N-[(1R)-1-(4-fluorophenyl)ethyl]-N'-[(2S,3S)-3-hydroxy-4-{4-[(1S)-1-hydroxyethyl]-1H-1,2,3-triazol-1-yl}-1-phenylbutan-2-yl]-5-[methyl(methylsulfonyl)amino]benzene-1,3-dicarboxamide | C32 H37 F N6 O6 S | 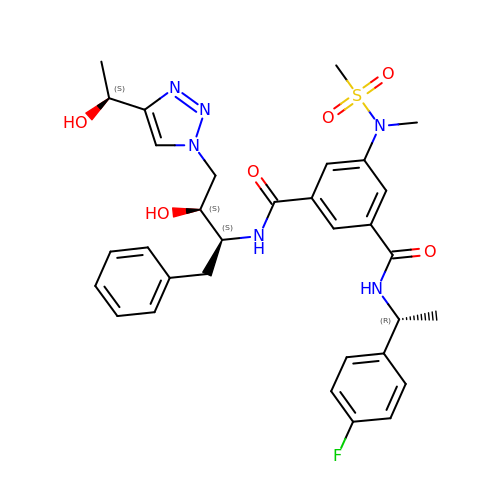CUYAHRWSXUTTQB-PELBXYKSSA-N N-(tert-butyl)-4-[5-(pyridin-2-ylamino)quinolin-3-yl]benzenesulfonamide | C24 H24 N4 O2 S | 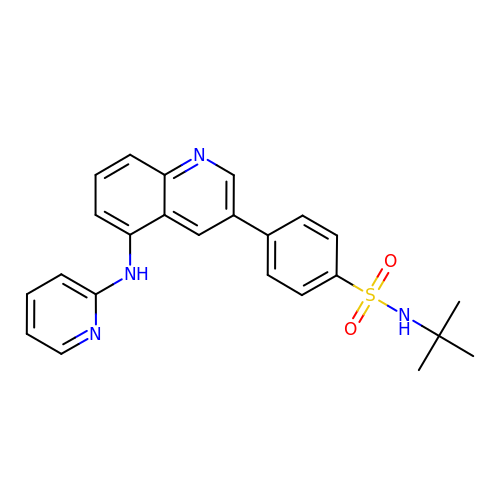GJTCKUKIFXWJKG-UHFFFAOYSA-N Sodium/proton exchanger 1 (NHE1) is an electroneutral secondary active transporter present on the plasma membrane of most mammalian cells and plays critical roles in regulating intracellular pH and volume homeostasis. Calcineurin B-homologous protein 1 (CHP1) is an obligate binding partner that promotes NHE1 biosynthetic maturation, cell surface expression and pH-sensitivity. We find that NHE1 assembles as a symmetrical homodimer, with each subunit undergoing an elevator-like conformational change during cation exchange. Each monomer is made up of a dimerization domain (TMs 1−3 and 7−10) and a core domain (TMs 4−6 and 11−13).

To investigate how the NHE1-CHP1 complex is activated by protonation, we prepared a sample at pH 6.5 as well as in the presence of 150-mM NaCl. Three-dimensional reconstruction of the corresponding NHE1-CHP1Na/6.5 dataset was similar to the NHE1-CHP1Na/7.5 dataset, resulting in a 3.4-Å map for the transporter complex. Subsequent 3D reconstruction focusing on this class without an imposed symmetry yielded a 4.0-Å EM map. Two helices were observed in the cytoplasmic region of the NHE1 protomer, termed HC1 and HC2. Whereas HC1 shows extensive interactions with CHP1, HC2 is amphipathic and presumably binds to the membrane surface. In the NHE1-CHP1Na/6.5 complex, HC1 and HC2 helices are perpendicular to each other. Moreover, the two CHP1 molecules reside at opposite ends of the rectangular-shaped NHE1 dimer, by interacting with IL6, HC1, and HC2, resulting in an ~30o angle between the CHP1 molecule and the membrane plane. We hypothesize that absence of the HC3 helices in the NHE1-CHP1Na/6.5 complex model is caused by the splay-opened CHP1, thus releasing the HC3 helices from the TMD dimer. A large funnel between the dimerization domain and the core domain in each protomer is accessible only from the intracellular side, indicating that in both pH conditions the NHE1-CHP1 complex adopts an inward-facing conformation. In the context of inward-facing NHE1-CHP1Na/7.5 and NHE1-CHP1Na/6.5 complexes, the CHP1 molecule exhibits high mobility relative to the NHE1 dimer, resulting in featureless CHP1 density in the EM maps.

>[2x]KAFPVLGIDYTHVRTPFEISLWILLACLMKIGFHVIPTISSIVPESCLLIVVGLLVGGLIKGVGETPPFLQSDVFFLFLLPPIILDAGYFLPLRQFTENLGTILIFAVVGTLWNAFFLGGLMYAVCLVGGEQINNIGLLDNLLFGSIISAVDPVAVLAVFEEIHINELLHILVFGESLLNDAVTVVLYHLFEEFANYEHVGIVDIFLGFLSFFVVALGGVLVGVVYGVIAAFTSRFTSHIRVIEPLFVFLYSYMAYLSAELFHLSGIMALIASGVVMRPYVEANISHKSHTTIKYFLKMWSSVSETLIFIFLGVSTVAGSHHWNWTFVISTLLFCLIARVLGVLGLTWFINKFRIVKLTPKDQFIIAYGGLRGAIAFSLGYLLDKKHFPMCDLFLTAIITVIFFTVFVQGMTIRPLVDLLAVKKKQETKRSINEEIHTQFLDHLLTGIEDICGHYGHHHWKDKLNRFNKKYV;>DEELEEIKKETGFSHSQITRLYSRFTSLDKGENGTLSREDFQRIPELAINPLGDRIINAFFPEGEDQVNFRGFMRTLAHFRPIEDNEKSKDVNGPEPLNSRSNKLHFAFRLYDLDKDEKISRDELLQVLRMMVGVNISDEQLGSIADRTIQEADQDGDSAASFTEFVKVLEKVDVEQKMSIRFLH[2x]>[2x]ALTRNLHPIGKIAITSVHLKLPILKGLSNDNLSAGAGTMKADQKMGEGNYALAGHYMTNQG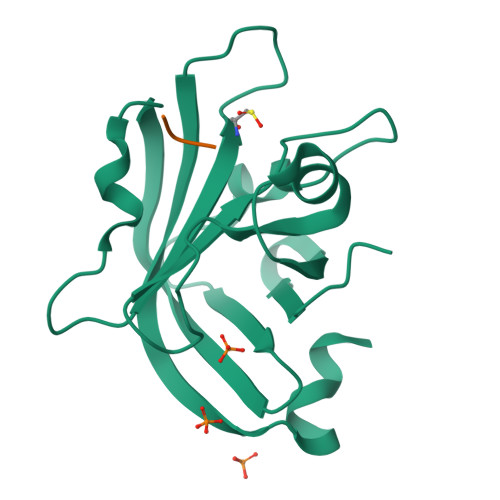ILFSPLKNVQTGDTVAITNMKKVYTYKVTTKQIVNETQVQWIDDVAGKKLITLVTCASPTEGEVDRIIVQGELQSVKKANQKNLKIFL;>ALT[2x]> MNDIAHNLAQVRDKISAAATRCGRSPEEITLLAVSATKPASAIAEAIDAGQRQFGENYVQEGVDKIRHFQELGVTGLEWHFIGPLQSNKSRLVAEHFDWCHTIDRLRIATRLNDQRPAELPPLNVLIQINISDENSKSGIQLAELDELAAAVAELPRLRLRGLMAIPAPESEYVRQFEVARQMAVAFAGLKTRYPHIDTLSLGMSDDMEAAIAAGSTMVRIGTAIFGARDYSKK

The pyridoxal 5′‐phosphate (PLP) homeostasis protein (PLPHP) is a ubiquitous member of the COG0325 family with apparently no catalytic activity. Although the actual cellular role of this protein is unknown, it has been observed that mutations of the PLPHP encoding gene affect the activity of PLP‐dependent enzymes, B6 vitamers and amino acid levels. Here we report a detailed characterization of the Escherichia coli ortholog of PLPHP (YggS) with respect to its PLP binding and transfer properties, stability, and structure. YggS binds PLP very tightly and is able to slowly transfer it to a model PLP‐dependent enzyme, serine hydroxymethyltransferase.

We serendipitously discovered that the K36A variant of YggS, affecting the lysine residue that binds PLP at the active site, is able to bind PLP covalently. This observation led us to recognize that a number of lysine residues, located at the entrance of the active site, can replace Lys36 in its PLP binding role.>[2x]SSIMKILLIGDVGVGKSCLLVRFVEDKFNPSFITTIGIDFKIKTVDINGKKVKLQLWDTAGQERFRTITTAYYRGAMGIILVYDVTDERTFT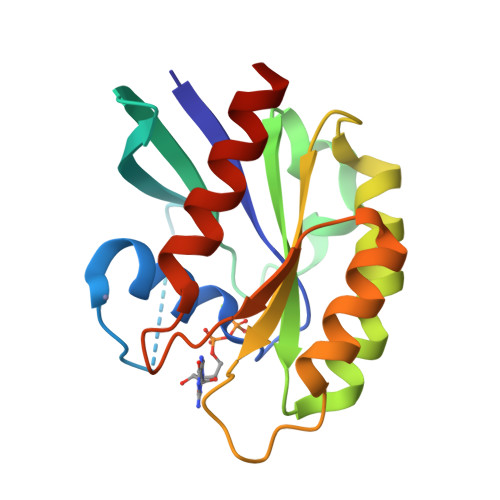NIKQWFKTVNEHANDEAQLLLVGNKSDMETRVVTADQGEALAKELGIPFIESSAKNDDNVNEIFFTLAKLIQEKIDSN> GGMAGQNPNMDQFEAYFKRADLDGDGRISGAEAVGFFQGSGLSKQVLAQIWSLSDRSHSGFLDRQNFYNSLRLVTVAQSKRDLTPEIVNAALNTPAAAKIPPPKINLSA

In contrast to animals and yeasts, CME in plants depends on the TPLATE complex (TPC), an evolutionary ancient adaptor complex. In this study, we used a multidisciplinary approach to elucidate the structural and functional roles of the evolutionary conserved N-terminal Eps15 homology (EH) domains of the TPC subunit AtEH1/Pan1. AtEH/Pan1 and Pan1p proteins are both hallmarked by the presence of two EH domains at their N-terminus. In conclusion, our parallel structural and functional comparison of the EH domains of AtEH/Pan1 revealed two divergent EH domains with differential, yet complementary functions.

EH1.1 consists of two EF-hands connected by two short antiparallel β-sheets. Anomalous scattering supports a calcium ion bound in a pentagonal-bipyramidal geometry in the loop of the first EF-hand. No anomalous scattering signal was detected in the second EF-hand loop, but electron density consistent with the coordination of a sodium ion was present. With respect to EH1.1, the NMR and X-ray structures agree very well with a RMSD of 1 Å. The major difference between the two domains is at the interaction interface of the N- and C-terminal ends. The hydrophobic core of EH1.1 is shielded by the proline-rich C-terminal loop, while in EH1.2, the proline-rich N-terminal loop takes over this function. On the one hand, EH1.1 coordinates the PA molecules by three main regions (residues around K42, residues around K78, and residues located at the C-terminus around K97). The N-terminal double NPF peptide of SCAMP5 was identified as a significant interactor of EH1.1. Bio-Layer Interferometry (BLI) confirmed the interaction between EH1.1 and a peptide derived from the N-terminus of SCAMP5 with a binding affinity (Kd) of 59 µM via steady-state kinetics. Mutating the conserved tryptophan to alanine (W49A) in EH1.1, and testing its binding capacity by BLI confirmed its essential role. We conclude that the N-terminal double NPF motif of SCAMP5 interacts preferentially with EH1.1, mediated via a hydrophobic interaction with the conserved tryptophan residue.> SMHPQAVAAVLPAGGCGERMGVPTPKQFCPILERPLISYTLQALERVCWIKDIVVAVTGENMEVMKSIIQKYQHKRISLVEAGVTRHRSIFNGLKALAEDQINSKLSKPEVVIIHDAVRPFVEEGVLLKVVTAAKEHGAAGAIRPLVSTVVSPSADGCLDYSLERARHRASEMPQAFLFDVIYEAYQQCSDYDLEFGTECLQLALKYCCTKAKLVEGSPDLWKVTYKRDLYAAESIIKERISQEICVVMDTEEDNKHVGHLLEEVLKSEL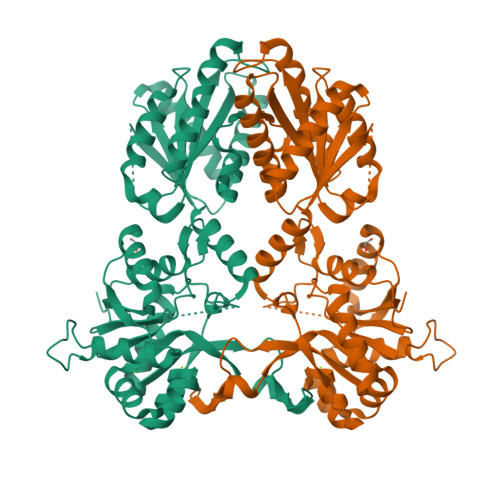NHVKVTSEALGHAGRHLQQIILDQCYNFVCVNVTTSDFQETQKLLSMLEESSLCILYPVVVVSVHFLDFKLVPPSQKMENLMQIREFAKEVKERNILLYGLLISYPQDDQKLQESLRQGAIIIASLIKERNSGLIGQLLIA>SGIVVSPILIPENQRQPFPRDVGKVVDSDRPEGSKFRLTGKGVDQDPKGTFRINENTGSVSVTRTLDRETIATYQLYVETTDASGKTLEGPVPL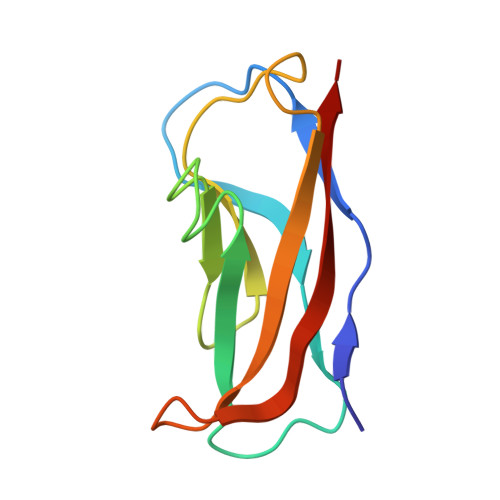EVIVID[2x]> MSSG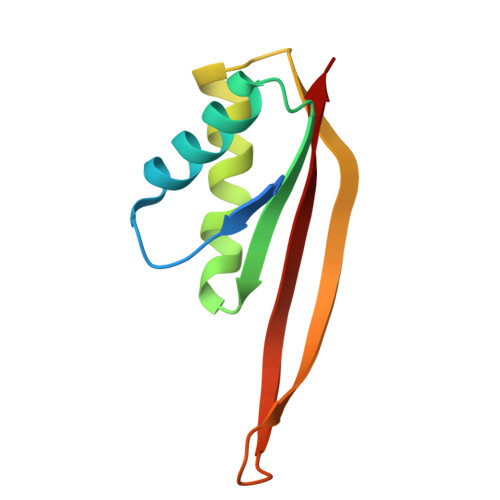TPTPSNVVLIGKKPVMNYVLAALTLLNQGVSEIVIKARGRAISKAVDTVEIVRNRFLPDKIEIKEIRVGSQVVTSQDGRQSRVSTIEIAIRKK> KSGDSSISISAIGNVDSPMIRITFQNQTEREFFLNKITDKAKSLGVNISTHPFEIKEPNMVLIKPSKYPDNKLGCYISKNKEIAINFGRTDFRDFVLSNLGVGSHLGTCPTKNET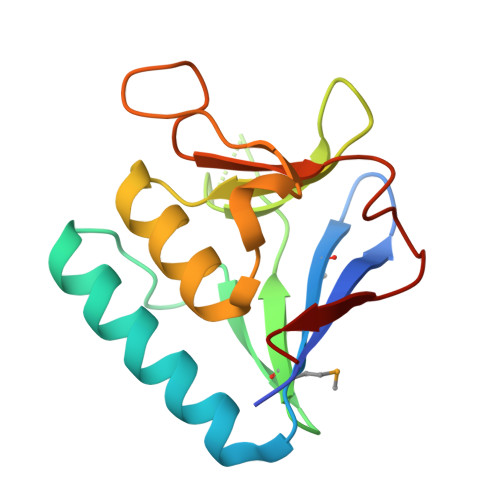GNDTFYFHQENLSLNGPALSVNTK> MALPQTVR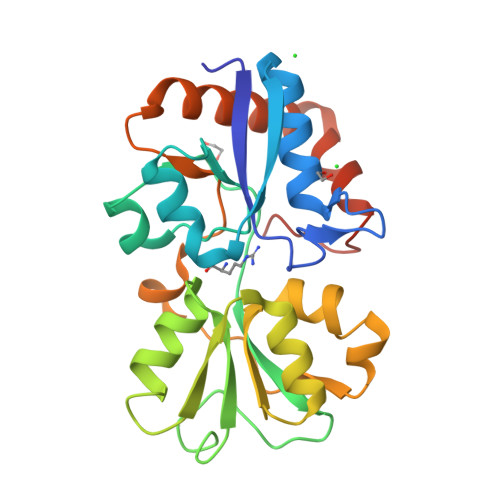IGTDTTYAPFSSKDAKGEFIGFDIDLGNEMCKRMQVKCTWVASDFDALIPSLKAKKIDAIISSLSITDKRQQEIAFSDKLYAADSRLIAAKGSPIQPTLESLKGKHVGVLQGSTAEAYANDNWRTKGVDVVAYANQDLIYSDLTAGRLDAALQDEVAASEGFLKQPAGKEYAFAGPSVKDKKYFGDGTGVGLRKDDTELKAAFDKALTELRQDGTYDKMAKKYFDFNVYGDKHHHHHH> MENSTSLKQEKENQEPGEAERLWQGESDVSPQEPGPPSPEYREEEQRTDTEPAPRMSPSWSHQSRVSLSTGDLTAGPEVSSSPPPPPLQFHSTPLNTETTQDPVAASPTEKTANGIADTGTPYSDPWESSSAAKQSTSHYTSHAEESTFPQSQTPQPDLCGLRDASRNKSKHKGLRFDLLQEEGSDSNCDPDQPEVGASEAAQSMLEVAIQNAKAYLLSTSSKSGLNLYDHLSKVLTKILDERPADAVDIIENISQDVKMAHFNKKLDTLHNEYEMLPAYEIAETQKALFLQGHLEGADSELEEEMAESSLPNVMESAYYFEQAGVGLGTDETYRVFLALKQLTDTHPIQRCRFWGKILGLEMNYIVAEVEFRDGEDEEEVEEEGIAEERDNGGSEAGEEEEEELPKSLYKAPQVIPKEESRTGANKYVYFVCNVPGRPWVRLPSVTPAQIVTARKIKKFFTGRLDA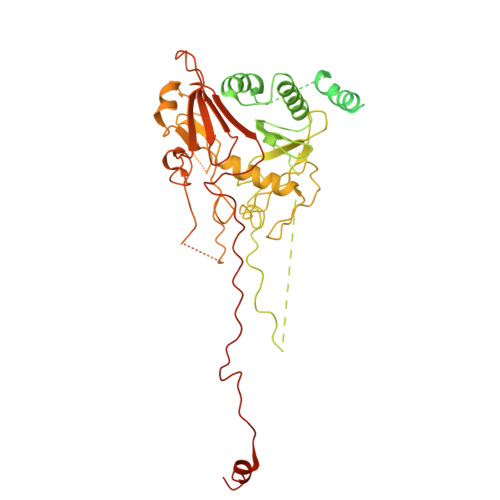AVISYPPFPGNESNYLRAQIARISAGTHVSPLGFYQFGEEEGEEEEVEGGRDSYEENPDFEGIQVIDLVESLSNWVHHVQYILPQGRCNWFNPIQKDEDEEEEEEEDEEKGEEPDYIEQEVGPPLLTPISEDLGIQNIPSWTTQLSSNLIPQYAIAVLRSNLWPGAYAFSNGKKFENFYIGWGHKYCVENYTPPSPPPVYQEYPSGPEITEMNDPSVEEEQAFRMTQEPVALSTEENEGTEDEDEDDED> SASAQQLAEELQIFGLDCEEALIEKLVELCVQYGQNEEGMVGELIAFCTSTHKVGLTSEILNSFEHEFLSKRLSKARHSTCKDSGHAGARDIVSIQELIEVEEEEEILLNSYTTPSKGSQKRAISTPETPLTKRSVSTRSPHQLLSPSSFSPSATPSQKYNSRSNRGEVVTSFGLAQGVSWSGRGGAGNISLKVLGCPEALTGSYKSMFQKLPDIREVLTCKIEELGSELKEHYKIEAFTPLLAPAQEPVTLLGQIGCDSNGKLNNKSVILEGDREHSSGAQIPVDLSELKEYSLFPGQVVIMEGINTTGRKLVATKLYEGVPLPFYQPTEEDADFEQSMVLVACGPYTTSDSITYDPLLDLIAVINHDRPDVCILFGPFLDAKHEQVENCLLTSPFEDIFKQCLRTIIEGTRSSGSHLVFVPSLRDVHHEPVYPQPPFSYSDLSREDKKQVQFVSEPCSLSINGVI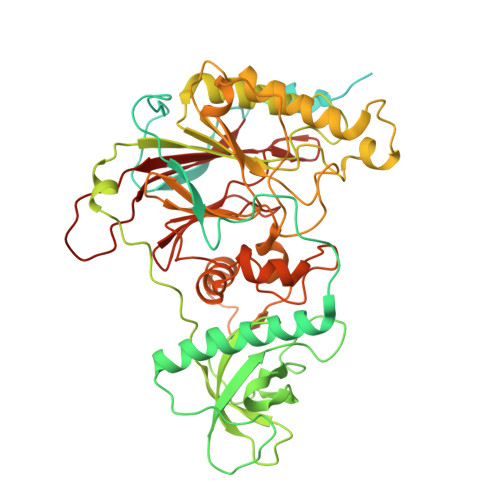FGLTSTDLLFHLGAEEISSSSGTSDRFSRILKHILTQRSYYPLYPPQEDMAIDYESFYVYAQLPVTPDVLIIPSELRYFVKDVLGCVCVNPGRLTKGQVGGTFARLYLRRPAADGAERQSPCIAVQVVRI> MDNSNGIHYIELTPNPIRFDAVSQLTNVFFDDSNKQIFAVRSGGATGVVVKGPGSPDDVVISFCMSDRGGAIRSIKFSPDNQILAVQRKENSVEFICFQGDQPLLQDIITHQVKTLIHGFVWVHNREVALISNTGVEVYTVVPEKRQVRSVKSLSIGIKWFAWCCDANVALLCTSEGNSLIPVLVKQKVITKLPKVDLGNPSRDVQESKVTLGQVYGVLAVLILQSNSTTGLMEVEVHLLNGPGLAPRKCHVLRLSLLGRFAINTVDNLIVVHHQASGTSLLFDISLPGEVINEITYHTPITPGRSIKPFGLKLPSLSPDGQILQCELYSTHWVLFQPNIVIDAKLGCMWFLNLCIEPLCQLISDRIRLTEFLLQRSNGKQMLLKVIGQLVDDQYKGTLLPVLETIFSRINKIYASWVQLELQNQTAQPSNVKTTTLKQSTP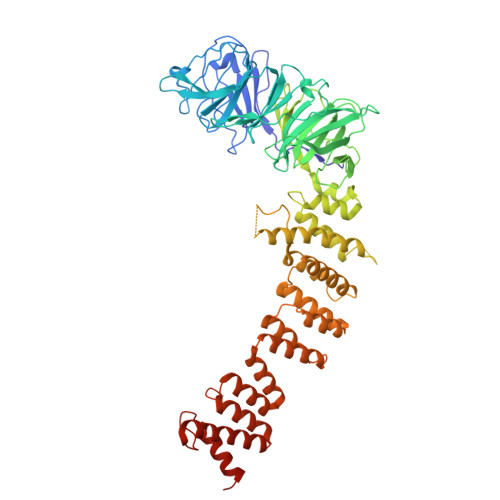PIVLIEQLDMVQIFQRIARRPYTESILMLYLQSLNKFNIAAQEELSKMIISELISNRSFDTLRRLVSYSMLLESKSVACFLLSHSNVDTAISQVAIDMLGRIEAHEIIIEVMLGQGKVIDALRLAKNSMGLEKVPARKFLEAAHKTKDDLIFHSVYRFFQMRNLKLYETLSFPKAEQCTEFIQHYNNTFPADNPTRQPVS>[2x]IR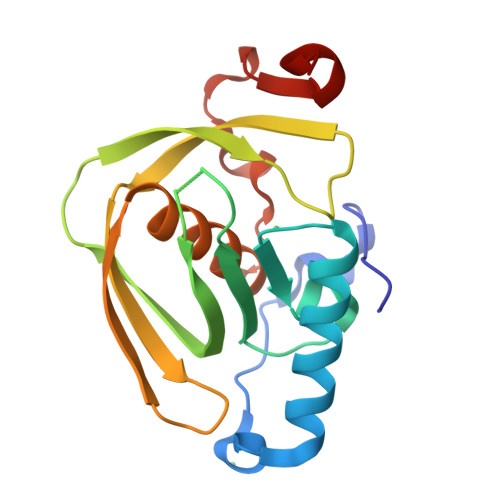EILKMGDERLLRIAQPVPSELLGSEELQRLIDDMFETMHHVGGVGLAAPQIGVDLQLVIFGFERSERYPDAPAVPPTILLNPRITPLDDEMEEGWEGCLSVPGLRGAVSRHRRIRYQGLDPQGQPIDRSVEGFHARVVQHECDHLIGRLYPSRITDFSKFGFTEVLFPD>MTDTYLHETLVFDNKLSYIDNQRDTDGPAILLLPGWCHDHRVYKYLIQELDADFRVIVPNWRGHGLSPSEVPDFGYQEQVKDALEILDQLGVETFLPVSHSHGGWVLVELLEQAGPERAPRGIIMDWLMWAPKPDFAKSLTLLKDPERWREGTHGLFDVWLDGHDEKRVRHHLLEEMADYGYDCWGRSGRVIEDAYGRNGSPMQMMANLTKTRPIRHIFSQPTEPEYEKINSDFAEQHPWFSYAKLGGPTHFPAIDVPDRAAVHIREFA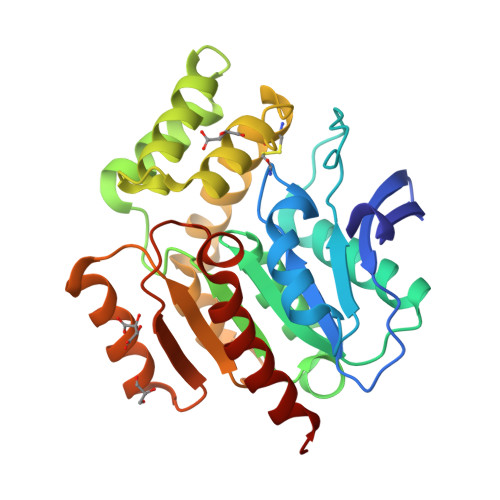TAIRQGQ[4x]(2S)-N,2-dimethyl-N-(propan-2-yl)morpholine-4-sulfonamide 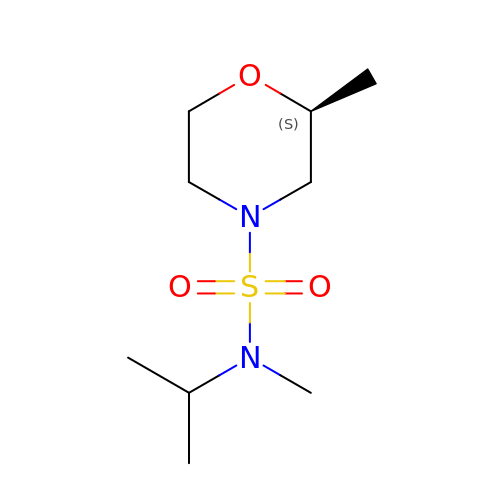| C9 H20 N2 O3 S | XYVINBFQYYSZBX-VIFPVBQESA-N3'-azido-3'-deoxythymidine | C10 H13 N5 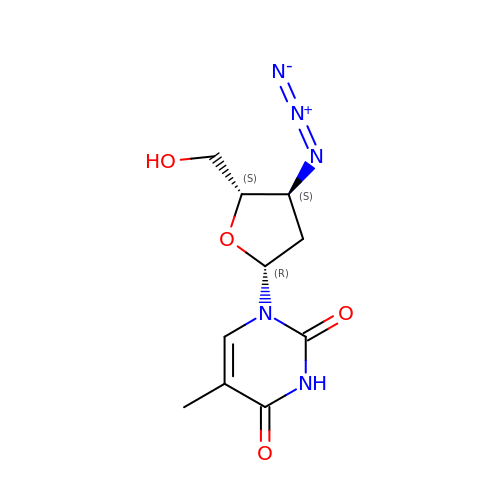O4 | HBOMLICNUCNMMY-XLPZGREQSA-N Amide synthases catalyze the formation of macrolactam rings from aniline-containing polyketide-derived seco-acids as found in the important class of ansamycin antibiotics. A key enzyme is the amide synthase ShGdmF (hereafter abbreviated as GdmF), which is not part of the PKS and is thought to catalyze the release of the ketide chain from the acyl carrier protein (ACP) domain of the last module 7 of the polyketide synthase. The overall folding of GdmF largely resembles the common architecture of its NAT analog, revealing a three-domain architecture with an N-terminal α-helical bundle (domain I, residues 1–88), a β-barrel (domain II, residues 89–185), and a C-terminal α/β-lid (domain III, residues 211–257), the latter being connected to domain II via an interdomain region (residues 186–210). The catalytic triad (Cys73-His111-Asp126 in GdmF) is highly conserved with an rmsd of 0.04 Å compared to the catalytic domain of MlNAT1 and is buried deep in the large active site cleft between domains II and III.

The substrate-bound protein structures agree well with the ligand-free structure of GdmF, with rmsd values between 0.05 and 0.137 Å for all backbone atoms, indicating only minor spatial changes within the subdomains upon substrate binding. To our surprise, we could not find electron density for the different thioester groups in any of these structures, but we found densities for the cleaved SNAC or pantetheine groups, instead. The SNAC and pantetheine groups are deeply embedded in the wide active site cleft, with the sulfur atom of the sulfhydryl group at a distance of only about 2 Å away from the reactive cysteine Cys73. GdmF, therefore, appears to be capable of directly binding SNAC and pantetheine thioesters and catalyzing the first step of macrolactamization, i.e., initiating nucleophilic attack of the activated ester carbon by the thiol group of Cys73 and thus cleavage of the thioester in the absence of arylamines. The bound SNAC and pantetheine co-substrates show conserved binding positions within the active site aligned with the β-strands of domains II and III. Two stabilizing interactions of the sulfur atom in the thioesters are observed with Tyr37 and His111. Although the orientation of the SNAC units within the hydrophobic active site cleft is the same for the different thioester derivatives, two alternative conformations of the acetamido group were observed, one of which forms an additional hydrogen bond to Gly110. This flexibility reflects the predominantly hydrophobic nature of the interactions with aliphatic and aromatic residues in the active site (Val72, Tyr74, Val98, Phe129, Pro130, and Phe210), and is consistent with mostly hydrophobic amino acids surrounding the catalytic triad in known NATs25. The SNAC (Kd = 1.16 mM) and pantetheine (Kd = 1.32 mM) prosthetic arms exerted comparable binding strengths in the low millimolar range.

> HHHHHHMFDVAKYLRRIGVEGTPPPTLDTLRHLHKRHLMAVPYDNSTAPDRLPASRHLTNVPLDLVFGHVVTEGHGGVCYELNRLFHTLLAELGYDVRMVAAAVRQANGTFGPEREHTFDLVHLDGRTHLVDVGFPGPSYSEPLYLSEEEQHQYGCSYRVTEHDGYRVVERRPKGSDWQPVYRFRPELADPSGWDAVRLDSLDDYAQDSVLAGTTFRSRATDNGKIVLIGRRYFTVEDGVERTKVLVKADEFQDVVDLILAGA> ANIVGGIEYSINNASLCSVGFSVTRGATKGFVTAGHCGTVNATARIGGAVVGTFAARVFPGNDRAWVSLTSAQTLLPRVANGSSFVTVRGSTEAAVGAAVCRSGRTTGYQCGTITAKNVTANYAEGAVRGLTQGNACMGRGDSGG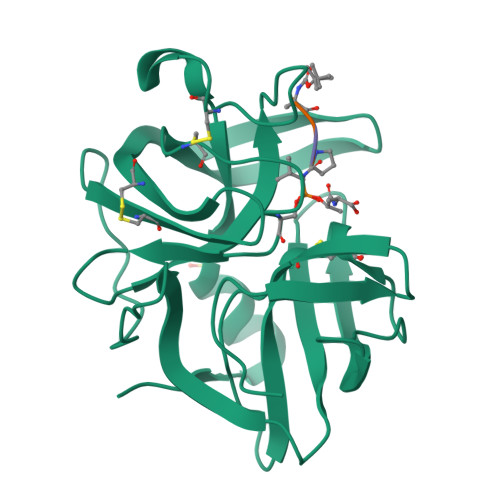SWITSAGQAQGVMSGGNVQSNGNNCGIPASQRSSLFERLQPILSQYGLSLVTG> APLVHHHHHHALANPAICRYPLGMSGGQIPDEDITASSQWSESTAAKYGRLDSEEGDGAWCPEIPVEPDDLKEFLQIDLHTLHFITLVGTQGRHAGGHGIEFAPMYKINYSRDGTRWISWRNRHG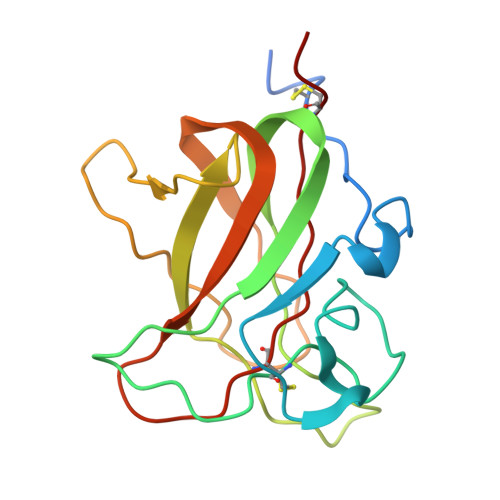KQVLDGNSNPYDIFLKDLEPPIVARFVRFIPVTDHSMNVCMRVELYGCVWLDG>MGSSHHHHHHSSGRENKYFQGHMRNVALITGITGQDGSYLAEFLLEKGYEVHGIVRRSSSFNTGRIEHLYKNPQAHIEGNMKLHYGDLTDSTCLVKIINEVKPTEIYNLGAQSHVKISFDLAEYTADVDGVGTLRLLDAVKTCGLINSVKFYQASTSELYGKVQEIPQKETTPFYPRSPYGAAKLYAYWIVVNFREAYNLFAVNGILFNHESPRRGANFVTRKISRSVAKIYLGQLECFSLGNLDAKRDWGHAKDYVEAMWLMLQNDEPEDFVIATGEVHSVREFVEKSFLHIGKTIVWEGKNENEVGRCKETGKVHVT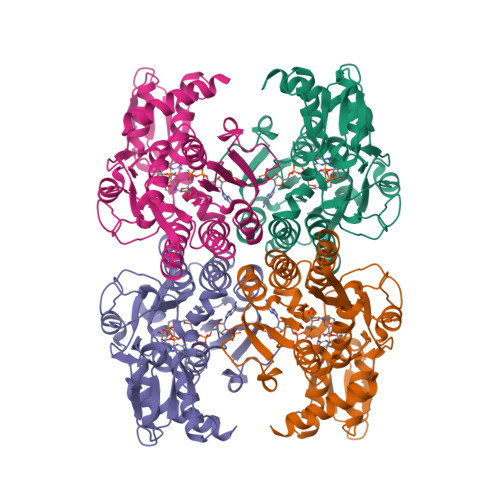VDLKYYRPTEVDFLQGDCTKAKQKLNWKPRVAFDELVREMVHADVELMRTNPNAGS[4x]> MMTGQVPILVLKEGTQREQGKNAQRNNIEAAKAIADAVRTTLGPKGMDKMLVDSIGDIIISNDGATILKEMDVEHPTAKMIVEVSKAQDTAVGDGTTTAVVLSGELLKQAETLLDQGVHPTVISNGYRLAVNEARKIIDEIAEKSTDDATLRKIALTALSGKNTGLSNDFLADLVVKAVNAVAEVRDGKTIVDTANIKVDKKNGGSVNDTQFISGIVIDKEKVHSKMPDVVKNAKIALIDSALEIKKTEIEAKVQISDPSKIQDFLNQETNTFKQMVEKIKKSGANVVLCQKGIDDVAQHYLAKEGIYAVRRVKKSDMEKLAKATGAKIVTDLDDLTPSVLGEAETVEERKIGDDRMTFVMGCKNPKAVSILIRGGTDHVVSEVERALNDAIRVVAITKEDGKFLWGGGAVEAELAMRLAKYANSVGGREQLAIEAFAKALEIIPRTLAENAGIDPINTLIKLKADDEKGRISVGVDLDNNGVGDMKAKGVVDPLRVKTHALESAVEVATMILRIDDVIASKKSTPPSGQGGQGQGMPGGGMPEY;> MIAGQPIFILKEGTKRESGKDAMKENIEAAIAISNSVRSSLGPRGMDKMLVDSLGDIVITNDGVTILKEMDVEHPAAKMMVEVSKTQDSFVGDGTTTAVIIAGGLLQQAQGLINQNVHPTVISEGYRMASEEAKRVIDEISTKIGADEKALLLKMAQTSLNSKSASVAKDKLAEISYEAVKSVAELRDGKYYVDFDNIQVVKKQGGAIDDTQLINGIIVDKEKVHPGMPDVVKDAKIALLDAPLEIKKPEFDTNLRIEDPSMIQKFLAQEENMLREMVDKIKSVGANVVITQKGIDDMAQHYLSRAGIYAVRRVKKSDMDKLAKATGASIVSTIDEISSSDLGTAERVEQVKVGEDYMTFVTGCKNPKAVSILVRGETEHVVDEMERSITDSLHVVASALEDGAYAAGGGATAAEIAFRLRSYAQKIGGRQQLAIEKFADAIEEIPRALAENAGLDPIDILLKLRAEHAKGNKTYGINVFTGEIEDMVKNGVIEPIRVGKQAIESATEAAIMILRIDDVI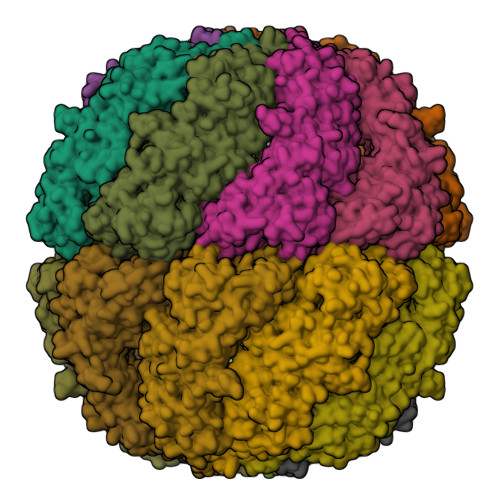ATKSSSSSSNPPKSGSSSESSED> GPMGNGMNKILPGLYIGNFKDARDAEQLSKNKVTHILSVHDSARPMLEGVKYLCIPAADSPSQNLTRHFKESIKFIHECRLRGESCLVHCLAGVSRSVTLVIAYIMTVTDFGWEDALHTVRAGRSCANPDVGFQRQLQEFEKHEVHQYRQWLKEEYG

DUSP22 is a small phosphatase containing 184 residues, and the sequence contains a catalytic domain as well as an N-terminal myristoylation site. This enzyme is broadly expressed in different tissues and plays important roles in the regulation of signaling pathways, such as inactivating the T cell receptor (TCR) signaling pathway, activating the JNK signaling pathway, and regulating the phosphorylation of focal adhesion kinase (FAK). The phosphatase domain of DUSP22 consists of five twisted β-sheets and six α-helices, and the structural scaffold is similar to that of DUSP3 (VHR), while DUSP22 does not contain an N-terminal α-helix surrounded by the N-loop. In this region, the catalytic activity is facilitated by C88 in the P-loop and D57 in the D-loop, and the hydrogen bonding network is formed by D57 in the D-loop, S93 in the P-loop, and N128 in the N-loop.

Structural alignment among N128A, N128D, and WT_VO4 revealed that N128 participated in forming the conformation of the D-loop. The negative charge from D128 in the N128D mutant induced charge repulsion against D57, which resulted in unclear electron density in the conformation of the D-loop and slightly shifted the N-loop. These results clearly indicated that the N128-D57 interaction anchored the D-loop and stabilized the conformation of the active site. N128A and N128D increased the KM more than 30 times, but the kcat values were different. N128D decreased the kcat by 16 times, while the kcat of N128A only decreased 2.5 times. Disruption of the DPN–triloop interaction by N128A and N128D critically decrease the catalytic efficiency by 100–500 times because it induces conformation changes in the D-loop and perturbs the conformation of the P-loop. In the N128D structure, the charge repulsion induces D57 to be unable to interact with S93 and substrate, which decreases the kcat.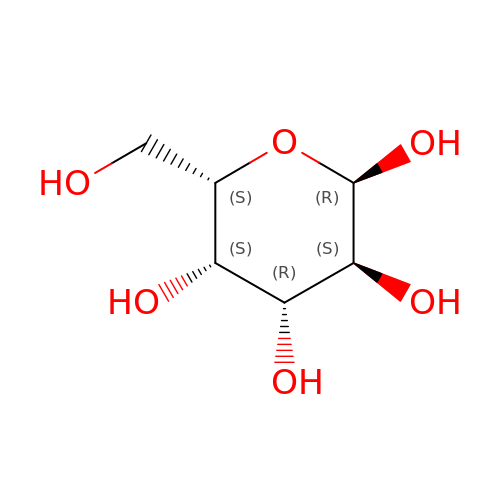alpha-L-galactopyranose | C6 H12 O6 | WQZGKKKJIJFFOK-SXUWKVJYSA-N> MSRLLALLALAPLLAGAAETTAPKPPSAFTVEAQRRVEAELPFADRADFERADRGLIRRPERLLIRNPDGSVAWQLGGYDFLLDGKPRDSINPSLQRQALLNLKYGLFEVAEGIYQVRGFDLANITFIRGDSGWIVVDTLTTPATARAAYELVSRELGERPIRTVIYSHAHADHFGGVRGLVEPQQVASGAVQIIAPAGFMEAAIKENVLAGNAMMRRATYQYGTQLPKGPQGQVDMAIGKGLARGPLSLLAPTRLIEGEGEDLVLDGVPFTFQNTPGTESPAEMNIWLPRQKALL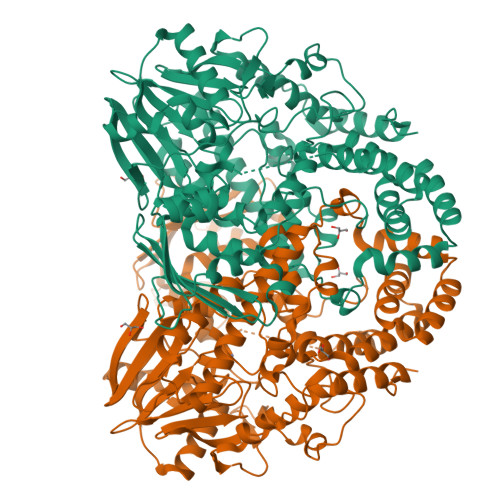MAENVVGTLHNLYTLRGAEVRDALGWSKYINQALHRFGRQAEVMFAVHNWPRWGNAEIVEVLEKQRDLYGYLHDQTLHLANQGVTIGQVHNRLRLPPSLDQEWYDRGYHGSVSHNARAVLNRYLGYYDGNPATLDPLSPEDSAGRYVEYMGGAERLLEQARASYARGEYRWVVEVVNRLVFAEPDNRAARELQADALEQLGYQAENAGWRNSYLSAAYELRHGVPRDQPTMKAGSADALAAMDTGLLFDYLGVRLDAGAAEGKALSINLRLPDIGENYLLELKNSHLNNLRGVQSEDAGQTVSIDRADLNRLLLKEVSAVRLVFEGKLKSSGNPLLLGQLFGMLGDFDFWFDIVTPAAKSEG>[4x]MSETPRLLFVHAHPDDESLSNGATIAHYTSRGAQVHVVTCTLGEEGEVIGDRWAQLTADHADQLGGYRIGELTAALRALGVSAPIYLGGAGRWRDSGMAGTDQRSQRRFVDADPRQTVGALVAIIRELRPHVVVTYDPNGGYGHPDHVHTHTVTTAAVAAAGVGSGTADHPGDPWTVPKFYWTVLGLSALISGARALVPDDLRPEWV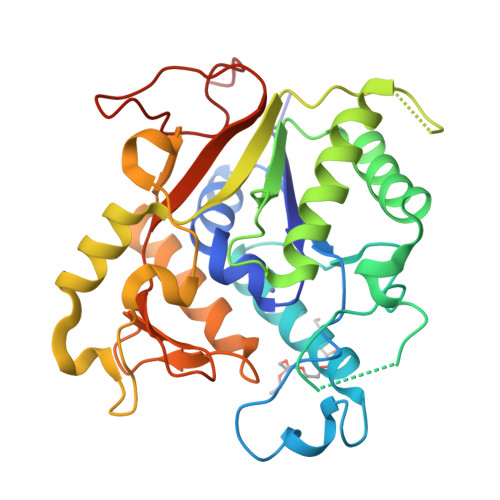LPRADEIAFGYSDDGIDAVVEADEQARAAKVAALAAHATQVVVGPTGRAAALSNNLALPILADEHYVLAGGSAGARDERGWETDLLAGLGFTASGT>[4x]SMQEGSLPDITIFPNSSLMISQGTFVTVVCSYSDKHDLYNMVRLEKDGSTFME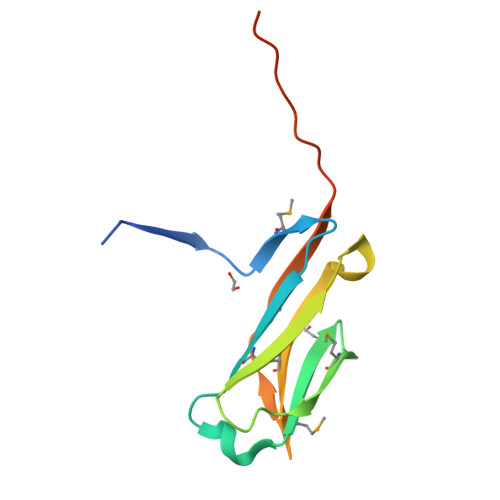KSTEPYKTEDEFEIGPVNETITGHYSCIYSKGITWSERSKTLELKVIKENVIQTPAPGPTSEHLG> ANTSSAYNSVYDFLRYHDRGDGLTVNGKTSYSIDQAAAQITRENVSWNGTNVFGKSANLTFKFLQSVSSIPSGDTGFVKFNAEQIEQAKLSLQSWSDVANLTFTEVTGNKSANITFGNYTRDASGNLDYGTQAYAYYPGNYQGAGSSWYNYNQSNIRNPGSEEYGRQTFTHKIGHALGLAHPGEYNAGEGDPSYNDAVYAEDSYQFSICSYWGENETGADYNGHYGGAPMIDDIAAIQRLYGANMTTRTGDSVYGFNSNTDRDFYTATDSSKA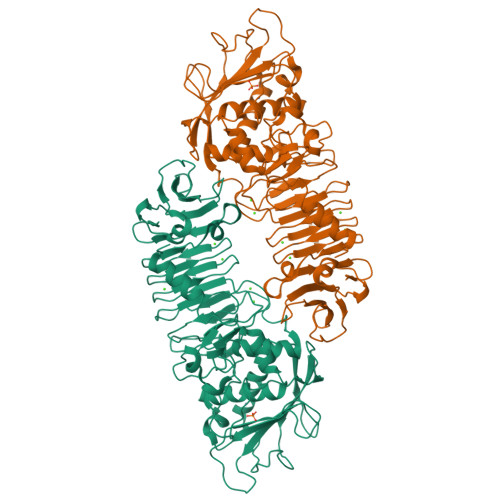LIFSVWDAGGTDTFDFSGYSNNQRINLNEGSFSDVGGLKGNVSIAHGVTIENAIGGSGNDILVGNSADNILQGGAGNDVLYGGAGADTLYGGAGRDTFVYGSGQDSTVAAYDWIADFQKGIDKIDLSAFRNEGQLSFVQDQFTGKGQEVMLQWDAANSITNLWLHEAGHSSVDFLVRIVGQAAQSDIIV>SVVIVGKISFCPKDVLGHGAEGTIVYRGMFDNRDVAVKRILPECFSFADREVQLLRESDEHPNVIRYFCTEKDRQFQYIAIELCAATLQEYVEQKDFAHLGLEPITLLQQTTSGLAHLHSLNIVHRDLKPHNILISMPNAHGKIKAMISDFGLCKKLAVGRHSFSRRSGVPGTEGWIAPEMLSEDCKENPTYTVDIFSAGCVFYYVISEGSHPFGKSLQRQANILLGACSLDCLHPEKHEDVIARELIEKMIAMDPQKRPSAKHVLKHPFFWSLE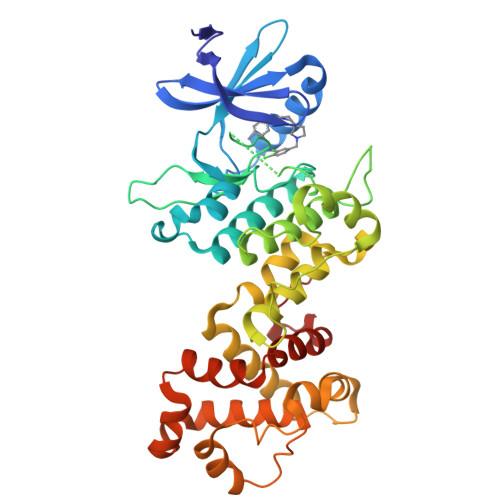KQLQFFQDVSDRIEKESLDGPIVKQLERGGRAVVKMDWRENITVPLQTDLRKFRTYKGGSVRDLLRAMRNKKHHYRELPAEVRETLGSLPDDFVCYFTSRFPHLLAHTYRAMELCSHERLFQPYYFHEPP[3x]>MKVLPKLALANLVCFTTLSVFAQPADPSGQQTSTNTSNLVTYLTNLGKYLGYDITQSSKAPNPPYSQLFNSNVVQLVQNYAYNTFLGAIPVDAMSQSLMNFVTDKVQGNSLINNLANTTFKYQNFSAPSSGADGKITANGLIDQSTASAQTPTTPGIFSAPQITTSGTYLNDPVSQAVFNILGTPDYSFCMDNEQKNWLPNCNLMYQNLVMQNVIGTLPPAQTSGSTPAFYSYKYNQPLISQLNSNSLIAPLLMDTSASQSGQDSGLTAKSQAQQALNFIRYASAQVTPPSLPKLSAYSELWNQATAKPNSAGYNEVQQKQAAATLSSYFNNLRVYAAQTSVGVSNLYYILSKRLPQNMSADQSNANITSQALNEFNMATRRLFDPTASNTPGQPNQQWIKQINDASPATVQKEIAILLAEINYQMYLDRQIQERILLTNSIMLLQNLKAAQPTADFSSQGSPSEQ[5x];>MNKLAITVLLCFFPALALAENGALSFAPPASDLSVVFLGNLFGVVDGVLHGTGSQIMGNMFGVFNSAVLALGGIIIMYTLMVSTMNTAHEGQMLGQKWSSIWIPLRSTFGLALLIPKASGYCMMQVFFMWVIVQGVGAADKIWEAALSYLNRGGVIIQAQADPTKSLQAAGSSSSGVAKGALTILGGQICMLGLQKQLQAQRDLYLSQSKSPPCGGNPTPEMNTFCRTAIPDFISTVNFVKKQNDDTPKDLTANQPASFELDMPNFDKSSPFYFLNGICGTVKWNNISALNSTNQSDNKGLVTVGGAGSNSSMGANSLNITSSQLQTARLSRAIAIQQMYVTLSTVAQVMVNNDPAFSTTTSTGNSKNDFSAIAKQQFGVPYKSSGEVCTEYQQVCQTWG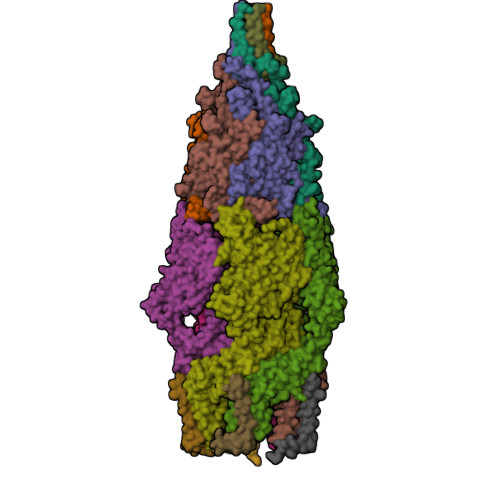SVPSSTGSTTGVLFNGTEFLGAINDYNGIMMPTLNLIRQATSKEFDKKSRDFIAEANAKGWIMAGSYFFDLVKLNGSATEFADQFDTGTGLDKSSFDPTQLTKPFGKTCQDPYSLLCTWFQNKSDKLIQIQSLIDGVPALGQDGVKQPDLSDNPQRQSVSGPLSSTVYGFVNNSMMVQLPGQPGIKPLTFANLINFKVDTSLYYMKHQDFDCGRVKILFFSFCLGRMMGDLFYNYVFRYVYNFFLAIFGEMINSIVMAFLMIPLQGMKDIFIVGVQTLTQPGINPIVALANMGTMYINFSGTLWLTLLNMAVVSSLIPLFGIFIFALIMMAMPLLMAWIGTMVSIGFVTAYYIPVLPYMIFTFGSFAWLIAVIEAMVAAPIVALGVTHPEGNEAFGKGEFAIMILVNVFLRPSLMIIGYIAAIALSYVGVWILNAGFDHAISYIQSDQGIETWEKGTSSNDAKRFFQSAGNWTGAKMDTSQWDNFKDKLTGDYQSTALEGGYTGWAGVYAFFFSILIYTSMYLIIVQKAFTLIAHLPDKVLRWIGGSPESFGQETMQWGEEAKGRVEKAGEATYGAEKAIGDKLGAKGQEMLGKLGPQAKKISENAGDVSGKGKNSGGSQTGPSSKPDTGQQLGGSDSGTPTSTPPPE[5x];>[5x]MASKKENLKSLFSNTRTRVIIIFTAALLIIAVVIGFFKIRGATTGSIAAAEVSTVPGGIQSIPGVLDPTAQYAKLQEEQNITQAQVAEKTGGSAIPTIIRTQALGEGVGVIGSQSGVGFAALAQEELGGPQRSLWIQELQDGSCSKSVITKVVNQGAQLTDLKAACSCVQLKDSGYGLQELEQVCECKELKSAGYNARQLKEAGYSAGRLRNCGFDACELRNAGFTAQEMKDGGFSDGELKGAGFSDAEIAKASGLPDGITADDVRKAGCGAAALAKLRQAGVSASAIRKISGCTAEQLKAAGYTAKELKDAGFSAADLRRAGFSAAELKDAGFTARDLLNAGFTPADLAKAGFSDAQIKAAQAELPPGITPQDVKNAGCDVEALKKEREAGVSAALIRQYAGCSAQALKAAGFTDADLANAGFTPAQISAATPLSDAEIKAAGCDPDKLKKLFSAGVSAKRIKELNGCSAEALKAAGYDAQSLLAAGFTPQELLAAGFTPKQLEDAGLNPVSIIADGRVADCSVESLKKARAAGVSALTIKQTLGCSAAALKAAGYTAKELKDAGFTAAELKAAGFSAKELKDAGFTAKELRDAGFSAQELKDVGFSAKDLKDAGFSAAELKAAGFTAAQLKAAGFSAKDLKDAGFSAAELKAAGFSAKELKDAGFSASDLKNAGFSAKELKDAGFSASDLKSAGFSASELKNAGYSADELKKAGYTSAELRNAGFSPQESAVAGLQGPDLQQLDSSITGIPSIPGATPRPTTSDAASSAEQLQAILQKQNEQLAEQKYQQEIQQRTSDMLTAATQLVQDWKQVETQVYTEGTEETKTSGGESAVPGTGTGTGSNNQPVDQGAVSAQNQAIIKTGDIMFAVLDTSVNSDEPGPILATIVTGKLKGSKLIGSFNLPSNADKMVITFNTMSIPGAEKTISISAYAIDPNTARTALASRTNHHYLMRYGSLFASSFLQGFGNAFQSANTTITIGGTGGGNNITVANGVGRSTLENAVIGLATVGKAWSQQAQQLFNTPTTVEVYSGTGLGILFTQDVTTI>[4x]MATLAAPPPPLGESGNSNSVSRITREGKKITYKLNIMQQPKRARACGQGSKSHTD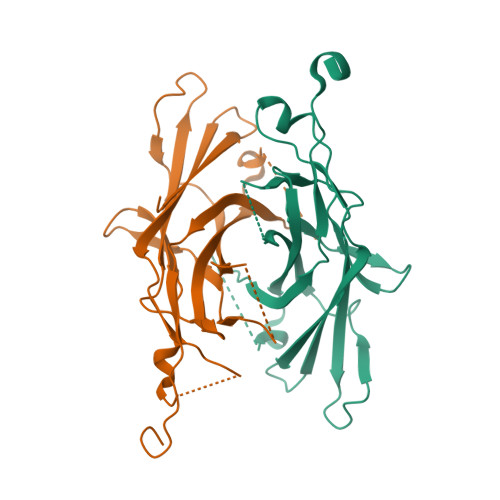RRPVDPPPVIELNIFESDPHDDSNKTDITFVYNANFFLFATLEPERPIATGKLMTNQGSPVLTGVPVAGVAYLDKPNRAGYFIFPDLSVRNEGSYRFSFHLFEQIKDPKDATEGTQPMPSPVPGKLSSPQEFLEFRLEVISNPFIVYSAKKFPGLTTSTPISRMIAEQG3'-deoxy-guanosine 5'-monophosphate | C10 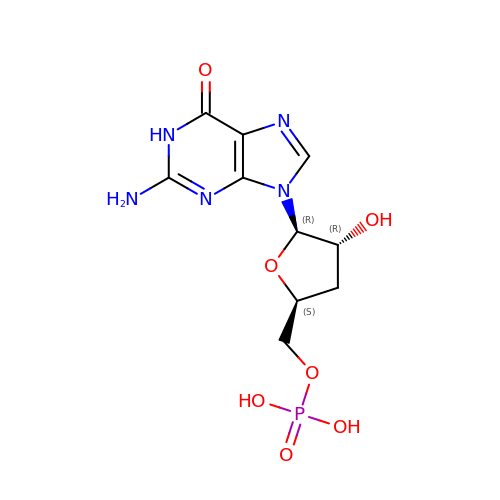H14 N5 O7 P | FDFODSATEZEUMJ-OBXARNEKSA-N By contrast, in vertebrates the clustered protocadherins (Pcdhs) provide analogous cell-surface diversity, but in this case generated through stochastic alternative promoter choice. Biophysical measurements with domain-deleted proteins showed that Pcdhs also interact in cis, through a membrane-proximal dimer interface involving extracellular cadherin domain 6 (EC6) and potentially EC5. The specificity-determining cell-cell recognition interface of Pcdhs involves domains EC1–4, as shown experimentally through mutagenesis analysis and suggested by mutation correlation analysis.

The γA isoform constructs—γA1EC1–4, γA4EC1–4, γA8EC1–4, γA9EC1–5—displayed dimer dissociation constants (KDs) of between 8.6 and 45.3 μM. Crystallization screening of these dimeric γ-Pcdh fragments yielded crystals of γA1EC1–4, γA8EC1–4, γA9EC1–5, γB2EC1–5, and γB7EC1–4, and their structures were determined by molecular replacement. X-ray diffraction by the γA9EC1–5 and γB7EC1–4 crystal form 1 crystals was significantly anisotropic and therefore the data was truncated using ellipsoidal limits for structure determination and refinement (Figure 1—source data 1 and Figure 1—figure supplement 2). The resolution of the final refined structures was 4.2 Å for γA1EC1–4, 3.6 Å for γA8EC1–4, 2.9/4.3/3.2 Å for γA9EC1–5, 3.5 Å for γB2EC1–5, 4.5/4.5/3.6 Å for γB7EC1–4 crystal form 1, and 3.1 Å for γB7EC1–4 crystal form 2. Unexpectedly the γA9EC1–5 crystal structure did not contain a trans dimer interaction in the crystal lattice. Given that γA9EC1–5 is a low micromolar dimer in solution, the monomeric arrangement in the crystal is likely an artifact of crystallization, perhaps due to the low pH (6.5) of the crystallization condition. We also found examples of small/large interacting residue pairs at the interface which showed correlated variations between isoforms such that heterophilic complexes would likely generate steric clashes: For example, EC1:EC4 residues 86 and 369 from γB isoforms, EC2:EC3 residues 125 and 253 of γB4 and γB5 (γB7 numbering), and EC1:EC4 residues 79 and 340 of γA8 and γA9.

> GQIRYSVPEETEKGYIVGNISKDLGLEPRELAERGVRIISKGKTQLFSLSPRSGSLVTAGRIDREELCAQSATCLLNFKVLVEDRVKLYGVEVEVVDINDNAPKFEAENLFVKISEIAAPGARYPLPEAVDPDVGINSLQSYQLSPNRHFSLHLQTGDDGTINPELVLERTLDREEEPTHHLVLTAYDGGNPRRSSTALIQVTVLDTNDNAPVFDQPVYRVKVLENVAPGTLLLTVRASDPDEGANGKVTYKFRKINEKHSLLFHLHENTGEMTVAKNLDYEECSLYEMEIQAEDGGGLKGRTKVVVMVEDVNDNRPEVTITSLFSPVREDAPPGTVILLFNAHDQDSGKNGQVVCSIQENPSFKLENSVDDYYRLLTAQILDREKASEYNITVTATDRGTPSMSTEVHITLYVADINDNPPAFSQTSYSVYLPENNPRGTSIFSVSAHDPDDEENAKVTYSLVENTIQGAPLSSYVSINSDTGVLYALQSFDYEQFQNLQMQVKASDNGHPPLSSNVSLSVFLLDQNDHHHHHHHH> GAHSERTFETAPSEIDADEVLEILSK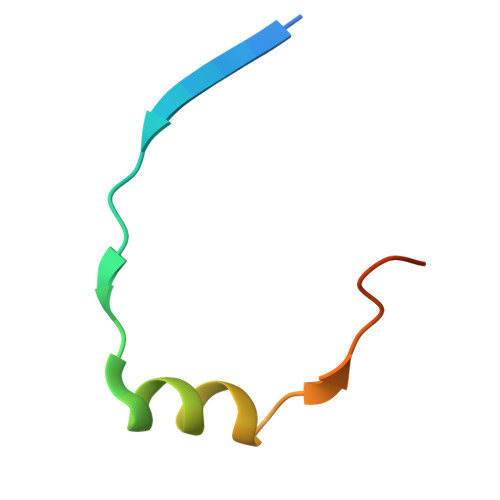SKPAPTHLTLER> QFSDMRI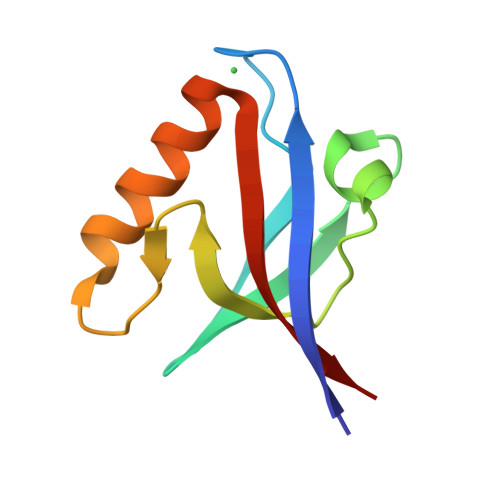SINQTPGKSLDFGFTIKWDIPGIFVASVEAGSPAEFSQLQVDDEIIAINNTKFSYNDSKEWEEAMAKAQETGHLVMDVRRYGK> GGLEKDFLPLSFGWFLTKKSSETLRKAGQVFLEELGNHKAFKKELRHFISGDEPKEKLELVSYFGKRPPGVLHCTTKFCDYGKAAGAEEYAQQEVVKRSYGKAFKLSISALFVTPKTAGAQVVLTDQELQLWPSDLDKPSASEGLPPGSRAHVTLGCAADVQPVQTGLDLLDILQQVKGGSQGEAVGELPRGKLYSLGKGRWMLSLTKKMEVKAIFTGYYG

2′,3′-cyclic nucleotide 3′-phosphodiesterase (CNPase) comprises 4% of total myelin protein in the central nervous system (CNS), being the most abundant CNS non-compact myelin protein4. CNPase consists of an N-terminal polynucleotide kinase-like domain10, a catalytic phosphodiesterase domain11, and a membrane-anchored C-terminal tail, which contains a cysteine residue that undergoes isoprenylation. The catalytic domain enables the rapid hydrolysis of nucleoside 2′,3′-cyclic phosphates to nucleoside 2′-phosphates. The CNPase catalytic site, lying in a groove between two lobes, has pseudo two-fold symmetry and contains two apposing His-X-Thr-X (X denotes a hydrophobic residue) motifs, characteristic for 2H phosphoesterases 113537.

Tyr168 interacts with the substrate ribose moiety through C-H…π hydrogen bonding. While the Y168A mutation decreases catalytic activity, Y168S retains it, albeit with an elevated KM compared to the wild-type enzyme. An increased KM, whilst retaining similar kcat, is an indication of decreased substrate binding affinity, with a minimal effect on actual catalysis. In the absence of the aromatic ring, the serine OH group appears to be enough to retain catalytic activity; this could be related to differences in water networks or overall dynamics in Y168A and Y168S. To further investigate the binding mode, we also attempted co-crystallization of CNPcat Y168S in the presence of 2′,3′-cAMP, but even residual ligand density in the active site could not be observed. In the mutants, the missing ion-dipole interaction between the Tyr168 hydroxyl group and the His230 imidazole ring apparently causes His230 and Ala/Ser168 to reposition in the active site by ~1 Å. Additionally, loop α3-β2 moves towards the active site by the same distance. These structural features suggest that Tyr168 also has a role in fine-tuning the active site conformation with its bulkiness.> SMDRRRFIKGSMAMAAVCGTSGIASLFSQAAFAADSDIADGQT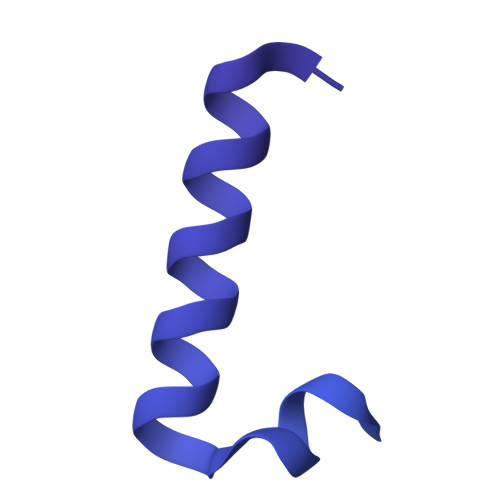QRFDFSILQSMAHDLAQTAWRGAPRPLPDTLATMTPQAYNSIQYDAEKSLWHNVENRQLDAQFFHMGMGFRRRVRMFSVDPATHLAREIHFRPELFKYNDAGVDTKQLEGQSDLGFAGFRVFKAPELARRDVVSFLGASYFRAVDDTYQYGLSARGLAIDTYTDSKEEFPDFTAFWFDTVKPGATTFTVYALLDSASITGAYKFTIHCEKSQVIMDVENHLYARKDIKQLGIAPMTSMFSCGTNERRMCDTIHPQIHDSDRLSMWRGNGEWICRPLNNPQKLQFNAYTDNNPKGFGLLQLDRDFSHYQDIMGWYNKRPSLWVEPRNKWGKGTIGLMEIPTTGETLDNIVCFWQPEKAVKAGDEFAFQYRLYWSAQPPVHCPLARVMATRTGMGGFSEGWAPGEHYPEKWARRFAVDFVGGDLKAAAPKGIEPVITLSSGEAKQIEILYIEPIDGYRIQFDWYPTSDSTDPVDMRMYLRCQGDAISETWLYQYFPPAPDKRQYVDDRVMS> MCCLYTSDVFFWSSLVVSPLPRIVRCVSAPQIRSIPCGSGDFSVMKRSLIARWQSGVHTPHGVVYRGAKMKNWPEQRIPENFKFTEEQRFRTKAIPRDVGTIPRNFVLGVLYRHQPCEVGGLWEHCTNDPEIVLDSKRHLREVLKQAREEGFVTFERDAISNEWLCFLTRERYEEVQRIVTAKSEAVDTHSGLRGAAATETSTYAEKFREMNVEAKEAHARRLEEEVANTTRYLRRFQQREIDYLPYTDLNGKVNFMWWYETRDVQQRADEVLTDSSSSKALAG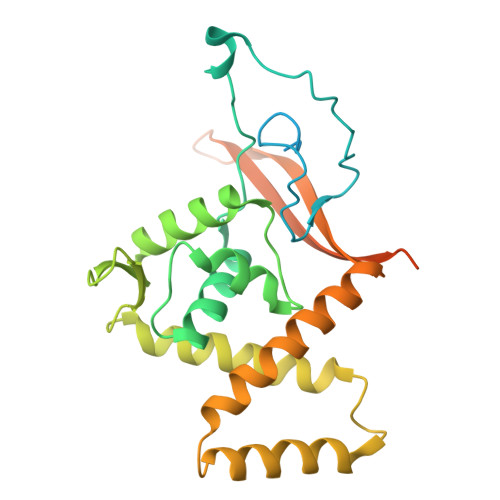EEEHKAGSQLEATTASTS Pinoresinol/lariciresinol reductase (PLR), an NADPH-dependent reductase, converts pinoresinol to lariciresinol and subsequently to secoisolariciresinol. Here, we present crystal structures of IiPLR1 from Isatis indigotica and pinoresinol reductases (PrRs) AtPrR1 and AtPrR2 from Arabidopsis thaliana, in the apo, substrate-bound and product-bound states. The crystal structures were captured in the apo, substrate-bound and/or product-bound forms. We found that, for all 16 structures we solved, each enzyme adopts a similar head-to-tail dimer conformation, strongly suggesting that each PLR/PrR functions as a homodimer, consistent with the literature that TpPLR1 exists as a dimeric entity in solution. Each structure contains a head-to-tail homodimer, and the catalytic pocket comprises structural elements from both monomers. β4 loop covers the top of the pocket, and residue 98 from the loop governs catalytic specificity.

Regarding the mechanism of the second catalytic step, we further compared the structures of IiPLR1_NAP_ + PIN, IiPLR1_NAP_-LAR and IiPLR1_NAP_-SEC, which revealed a similar mode for substrate/product binding. Furthermore, Leu46 (corresponding to Val46 in IiPLR1), His276 and Phe277 of AtPrR1 are positioned similar to the corresponding residues of IiPLR1 to effect substrate binding or product release, except that the β4 loops cover the substrate/product, which are disordered in the IiPLR1 structures.

>MRENNSGEKTRVLVVGGTGTMGRRIVRACLAEGHETYVLQQPETRVDIEKVQLLYSYKRLGARLIEASFSDHQSLVSAVKQVDIVVAAMSGVHFRSHSILVQLKLVEAIKEAGNIKRFLPSEFGMDPSRMGHAMPPGRETFDQKLEVRNAIEAAGIPHTYVVGACFAAYFAGNLSQMGTLIPPKKKVNIYGDGNVKVVYVDEDDIAEYTAKTLDDPRTINKTVYVRPTENVLTQMELVQIWEKLTGKELEKTNISANDFLADIEDKEIPHQAGLGHFYHIFYEGCLTDHEVGDDEEASKLYPDVKYTRMDEYLKIFL[6x]>[3x]MGSIGAASTEFCFDMFKELKVHHVNENIIYSPLSIISILSMVFLGARENTKTQMEKVIHFDKITGFGESLESQCGTSVSVHASLKDILSEITKPSDNYSLSLASKLYAEETYPVLPEYLQCIKELYKGSLETVSFQTAADQARELINSWVETQTNGVIKNFLQPGSVDPQTEMVLVDAIYFKGTWEKAFKDEDT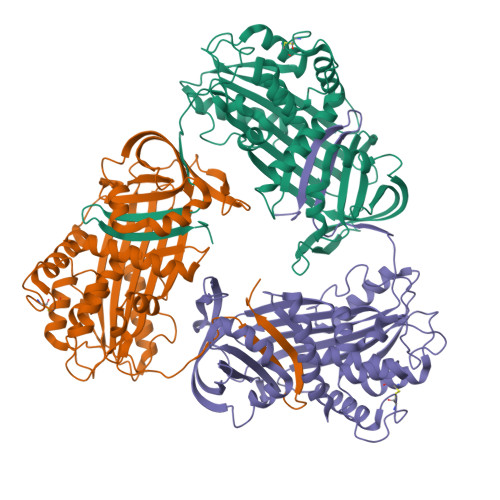QEVPFRITEQESKPVQMMYQAGSFKVATVAAEKMKILELPYASGELSMFVLLPDDISGLEQLETTISIEKLSEWTSSNMMEDRKMKVYLPHMKIEEKYNLTSVLVALGMTDLFSPSANLSGISTAQTLKMSEAIHGAYVEIYEAGSEMATSTGVLVEAASVSEEFRVDHPFLFLIKHNPSNSILFFGRCIFPHHHHHH>[5x]SNAMIIRPEQHWFLRLF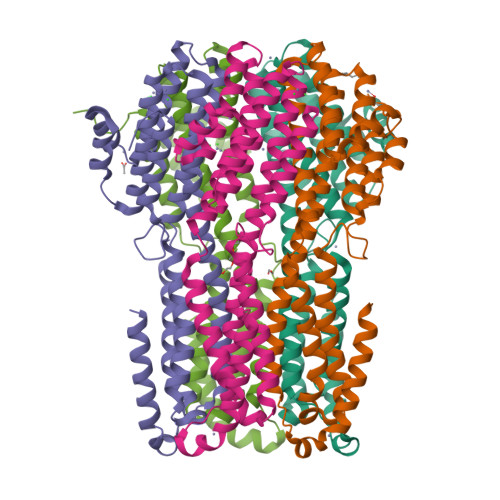DWHGSVLSKIIFRLLLNVLMSIIAIISYQWYEQLGIHLTVAPFSLLGIAIAIFLGFRNSASYSRFVEARNLWGTVLIAERTLVRQLRNILPAEHDAHRRIVSYLVAFSWSLKHQLRKTDPTADLRRLLAEERVTEILASSMPTNRILLLAGNEIGQLREAGKLSDITYGLMDNKLDELAHVLGGCERLATTPVPFAYTLILQRTVYLFCTLLPFALVGDLHYMTPFVSVFISYTFLSWDSLAEELEDPFGTAANDLPLNAMCNTIERNLLDMTGQHPLPE[2(FORMYL-HYDROXY-AMINO)-ETHYL]-PHOSPHONIC ACID | C3 H8 N O5 P 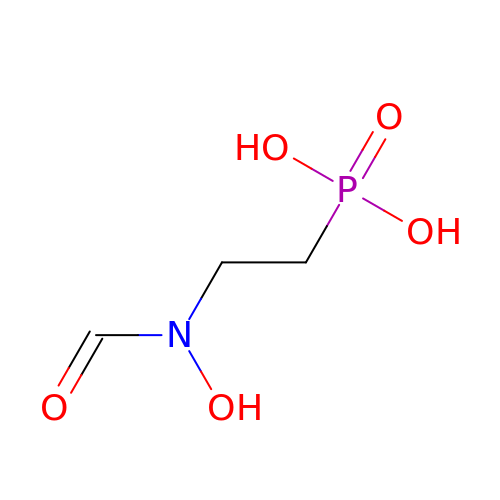| NBAIGNUEKZLOMI-UHFFFAOYSA-N>LKEKSWRDLSYLLKIKELKEAKKEFEKIFIEEKLREYDYDLKR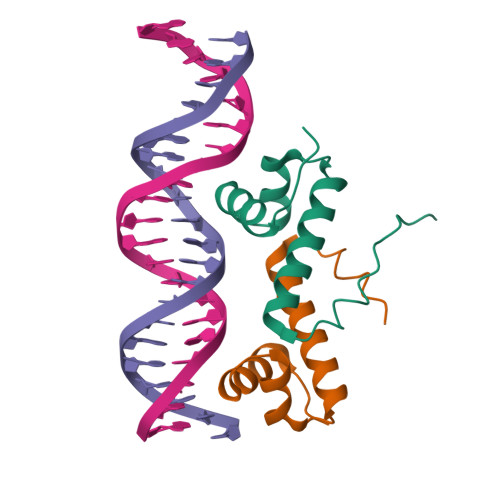TAEEIGIDLSNLYRKIKSLNIRVKSS[2x]>[8x]MSTDKITFLLNWQPTPYHIPIFLAQTKG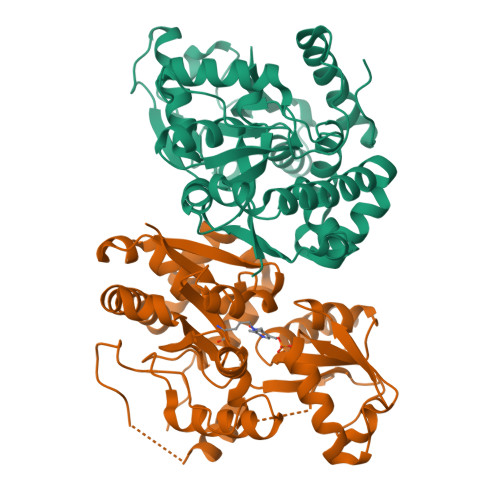YFKEQGLDMAILEPTNPSDVTELIGSGKVDMGLKAMIHTLAAKARGFPVTSVASLLDEPFTGVLYLKGSGITKSFQSLKGKKIGYVGEFGKIQIDELTKHYGMKPEDYTAVRCGMNVAKYIIEGKIDAGIGIECMQQVELEEYLAKQGRPASDAKMLRIDKLACLGCCCFCTVLYICNDEFLKKNPEKVRKFLKAIKKATDYVLADPVKAWKEYIDFKPQLNNDLSYKQYQRCYAYFSSSLYNVHRDWKKVTGYGKRLAILPPDYVSNYTNEYLSWPEPEEVSDPLEATRLMAIHQEKCRQEGTFKRLALPAHHHHHH>TDAPVSKASTVTGFGRGTNDVHLSGMSRISQAVLPAGTGTDGYVVVDATIVPDLLPRLGHAARIFQRYAVETLEFEIQPMCPANTGGGYVAGFLPDPTDNDHTFDA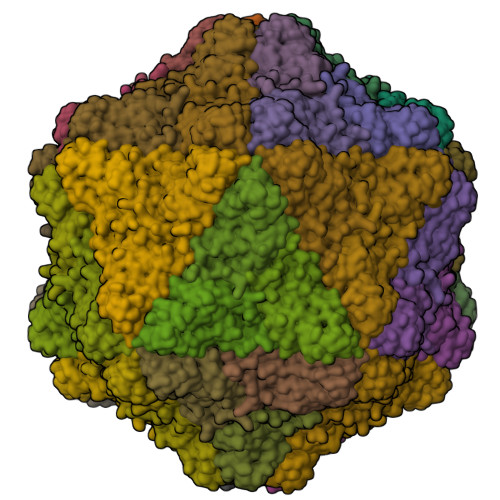LQATRGAVVAKWWESRTVRPQYTRTLLWTSSGKEQRLTSPGRLILLCVGNNTDVVNVSVLCRWSVRLSVPSLENPEE[60x]> MVFYSLVLVMKPRPRKYTSQALREIAVNIYNHG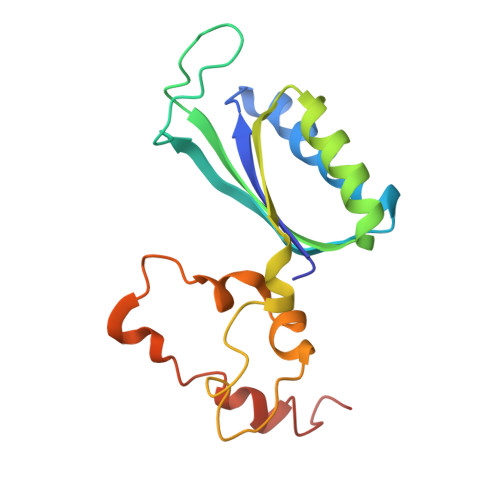GLIRKLSNEGILRPYSRFRDADNTAITYARYVTLQLDMGEEQMNKVEKIIREHADVNITLRLNNLERPTGVKHNQQSAAAYFPLDTFTRLEEEINWPPQVSGDVYEQLDMNWKEFSRTRWSNYLRN> HFTWDKYLKETCSVPAPVHCFKQS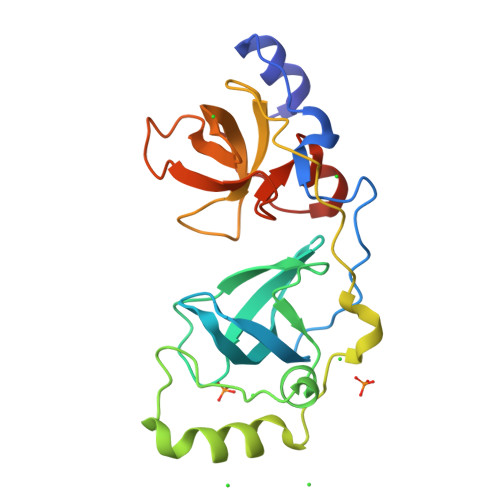YTPPSNEFKISMKLEAQDPRNTTSTCIATVVGLTGARLRLRLDGSDNKNDFWRLVDSAEIQPIGNCEKNGGMLQPPLGFRLNASSWPMFLLKTLNGAEMAPIRIFHKEPPSPSHNFFKMGMKLEAVDRKNPHFICPATIGEVRGSEVLVTFDGWRGAFDYWCRFDSRDIFPVGWCSLTGDNLQPPGTK>MADNQQRCELKLIASPGSWRLYSARKIDERFKSYEQKIFQRDRYTCQFCGFQARLYQDIVNLDGDYTNNRLSNLVTACCFCAQCFFVESVGVGGYGGGTLIYLPELTQAELNSLCHVLFCAITNDTGYKSSAQNIYRSFKFRSQIVEEKFGEGTSDPAIFGQLMIDSGVNSEEIREKLFKNIRLLPSRAKFRKQIEKWAASALEEIAD[11x];> RCELKLIASPGSWRLYSARKIDERFKSYEQKIFQRDRYTCQFCGFQARLYQDIVNLDGDYTNNRLSNLVTACCFCAQCFFVESVGVGGYGG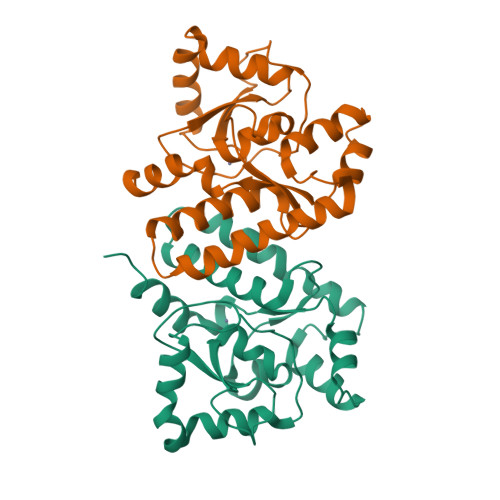GTLIYLPELTQAELNSLCHVLFCAITNDTGYKSSAQNIYRSFKFRSQIVEEKFGEGTSDPAIFGQLMIDSGVNSEEIREKLFKNIRLLPSRAKFRKQIEKWAAS>GAMGSESLSPGGPPGHPYQGEASTCWQLTVRVLEARNLRWADLLSEADPYVILQLSTAPGMKFKTKTLTDTSHPVWNEAFRFLIQSQVKNVLELSIYDEDSVTEDDICFKVLYDISEVLPGKLLRKTFSQSPQGEEELDVEFLMEETSDRPENLITNKVIVARELSCLDVHLDSTGSTAVVADQDKLELELVLKGSYEDTQTSFLGTASAFRFHYMAALETELSGRLRSSRSNGWNGDNSAGYLTVPLRPLTIGKEVTMDVPAPNAPGVRLQLKAEGCPEELAVHLGFNLCAEEQAFLSRRKQVVAKALKQALQLDRDLQEDEVPVVGIMATGGGARAMTSLYGHLLALQKLGLLDCVTYFSGISGSTWTMAHLYGDPEWSQRDLEGPIRYAREHLAKSKLEVFSPERLASYRRELELRAEQGHPTTFVDLWALVLESMLHGQVMDQKLSGQRAALERGQNPLPLYLSLNVKENNLETLDFKEWVEFSPYEVGFLKYGAFVPPELFGSEFFMGRLMRRIPEPRICFLEAIWSNIFSLNLLDAWYDLTSSGESWKQHIKDKTRSLEKEPLTTSGTSSRLEASWLQPGTALAQAFKGFLTGRPLHQRSPNFLQGLQLHQDYCSHKDFSTWADYQLDSMPSQLTPKEPRLCLVDAAYFINTSSPSMFRPGRRLDLILSFDYSLSAPFEALQQTELYCRARGLPFPRVEPSPQDQHQPRECHLFSDPACPEAPILLHFPLVNASFKDHSAPGVQRSPAELQGGQVDLTGATCPYTLSNMTYKEEDFERLLRLSDYNVQTSQGAILQALRTAL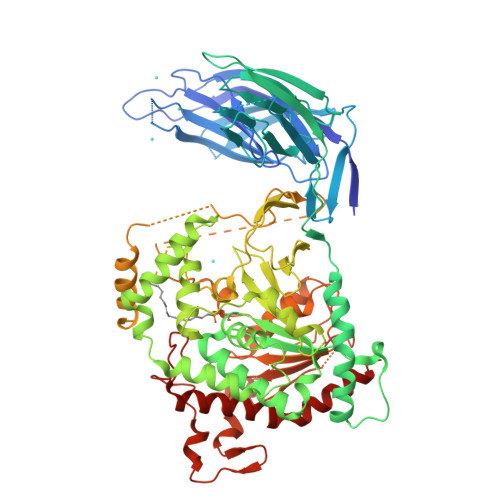KHRTLE[4x]> LHRASL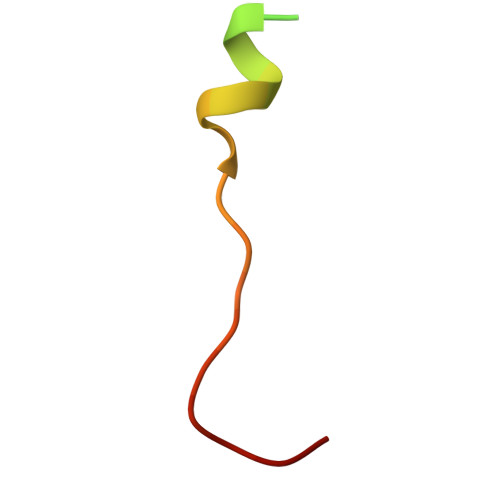FDHHELADYLISVGADINKID>GPLGSDNVPAPKHLTLERQLNKSVLIGWSPPEPVGYNLIDSYHVYVDGVLKVTVKANERTRALIEGVDSTRPHRISVRSVTQNRQTSRDAACTMIIGRDTAHLGPSAVRASHITCSSAVISWLPANSNHQHVVCVNNVEVRTVKPGMYRHTITGLAPSTQYRVTVRAKHLRAVGQHAANVGQTGGAGRPGQEEAPGAYADFRTLTKGLPDPPQEIQLEAGPQDGTILVTWQPVNRPTSTGPVTGYAVYADGKKVTDINSPTGDHALIDIGKLGVFNPRA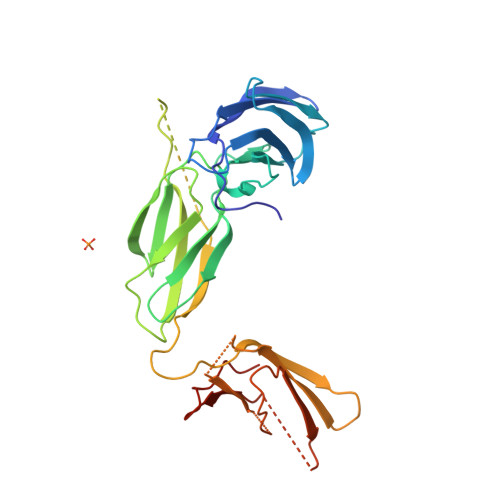VTIRTKSRDSQSADSAPILIPNTV[2x]Anaplastic lymphoma kinase (ALK) and the related leukocyte tyrosine kinase (LTK) are receptor tyrosine kinases (RTKs) that are activated by binding their cognate cytokines, ALKAL1 and ALKAL2 (also called FAM150A/B or AUGβ/α). Their signaling outputs elicit a range of pleiotropic activities in development and metabolism, and their dysregulated intracellular kinases are keenly pursued as therapeutic drug targets in various cancers. Recent structural studies revealed ALK/LTK-cytokine assemblies with distinct stoichiometries.

Here, we show based on reanalysis of the cryo-EM data deposited in EMPIAR-10930 that over half of the ALK-ALKAL2 particles in the dataset are classified into 2D and 3D classes obeying a 2:1 stoichiometry besides the originally reported structure displaying 2:2 stoichiometry. Unlike particles representing the 2:2 ALK-ALKAL2 complex, particles for the 2:1 ALK-ALKAL2 complex suffer severely from preferred orientations that resulted in cryo-EM maps displaying strong anisotropy. The combined use of Orientation Rebalancing in CryoSPARC and 3D refinement in RELION v5 with enabled Blush regularization, resulted in a final map at 3.2-Å resolution displaying an impressive improvement in isotropy, as evidenced by the 10-fold increase in the cFAR score, and overall interpretability. Most importantly, post-processing in RELION yielded a sharpened map with clear main chain connectivity and signal for most side chains, allowing complete model building of a 2:1 ALKTG-EGFL-ALKAL2 complex that includes the membrane-proximal EGFL-like domains of ALK. While the majority of the 2:1 ALKTG-EGFL-ALKAL2 cryo-EM map has a local resolution to better than 3.5-Å resolution, the C-terminal tips of the EGFL domains are only resolved at 4–4.5 Å resolution pointing to their inherent flexibility. Most importantly, though, this new structure is now the most complete ALK-ALKAL2 complex with 2:1 stoichiometry to date and agrees closely with the ALKTG-ALKAL2 with 2:1 stoichiometry reported by De Munck and colleagues featuring site 1 (ALK-ALKAL2), site 2 (ALK’-ALKAL2), and site 3 (ALK-ALK’) interaction interfaces. Accordingly, the root-mean-square deviation (r.m.s.d.) between these two structures is 1.3 Å over 675 aligned Cα-atoms. The site 2 interface present in the 2:1 ALK:ALKAL2 complex, but not in the 2:2 ALK-ALKAL2 complex, involves the α1 helix of ALKAL2 with a key histidine residue (H100) interacting with S737, Y739, and L760 of ALK’. Due to the asymmetric nature of the ALKAL2 monomer, the EGFL domain of the opposing ALK protomer (ALK’) in the 2:1 ALKTG-EGFL-ALKAL2 complex does not make any direct contacts at the “site 2” interaction with ALKAL2. As a result, the ALK’ EGFL domain is less resolved at its extremity due to increased flexibility, resulting in the absence of density for the minor β-hairpin in the cryo-EM map.

>[2x]GTAPKSRNLFERNPNKELKPGENSPRQTPIFDPTVHWLFTTCGASGPHGPTQAQCNNAYQNSNLSVEVGSEGPLKGIQIWKVPATDTYSISGYGAAGGKGGKNTMMRSHGVSVLGIFNLEKDDMLYILVGQQGEDACPSTNQLIQKVCIGENNVIEEEIRVNRSVHEWAGGGGGGGGATYVFKMKDGVPVPLIIAAGGGGRAYGAKTDTFHPERLENNSSVLGLNGNSGAAGGGGGWNDNTSLLWAGKSLQEGATGGHSCPQAMKKWGWETRGGFGGGGGGCSSGGGGGGYIGGNAASNNDPEMDGEDGVSFISPLGILYTPALKVMEGHGEVNIKHYLNCSHCEVDECHMDPESHKVICFCDHGTVLAEDGVSCIVSP;> GAEPREPADGQALLRLVVELVQELRKHHSAEHKGLQLLGRDYALGRAEAAGLGPSPEQRVEIVPRDLRMKDKFLKHLTGPLYFSPKCSKHFHRLYHNTRDCTIPAYYKRCARLLTRLAVSPVCMEDKQ> KRKDITLLNPIVRKFQYGQHTVTLETGMMARQATAAVMVSMDDTAVFVTVVGQKKAKPGQDFFPLTVNYQERTYAAGRIPGSFFRREGRPSEGETLIARLIDRPIRPLFPEGFVNEVQVIATVVSVNPQVNPDIVAMIGASAALSLSGIPFNGPIGAARVGYINDQYVLNPTQDELKESKLDLVVAGTEAAVLMVESEAQLLSEDQMLGAVVFGHEQQQVVIQNINELVKEAGKPRWDWQPEPVNEALNARVAALAEARLSDAYRITDKQERYAQVDVIKSETIATLLAEDETLDENELGEILHAIEKNVVRSRVLAGEPRIDGREKDMIRGLDVRTGVLPRTHGSALFTRGETQALVTATLGTARDAQVLDELMGERTDTFLFHYNFPPYSVGETGMVGSPKRREIGHGRLAKRGVLAVMPDMDKFPYTVRVVSEITESNGSSSMASVCGASLALMDAGVPIKAAVAGIAMGLVKEGDNYVVLSDILGDEDHLGDMDFKVAGSRDGISALQMDIKIEGITKEIMQVALNQAKGARLHILGVMEQAINAPRGDISEFAPRIHTIKINPDKIKDVIGKGGSVIRALTEETGTTIEIEDDGTVKIAATDGEKAKHAIRRIEEITAEIEVGRVYTGKVTRIVDFGAFVAIG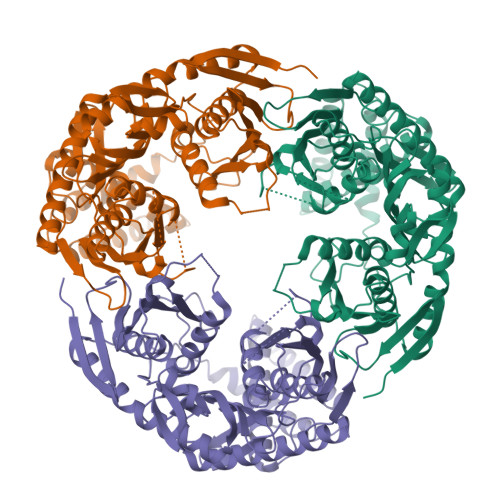GGKEGLVHISQIADKRVEKVTDYLQMGQEVPVKVLEVDRQGRIRLSIKEATEQSQPAAAPEAPAAEQGEHHHHHH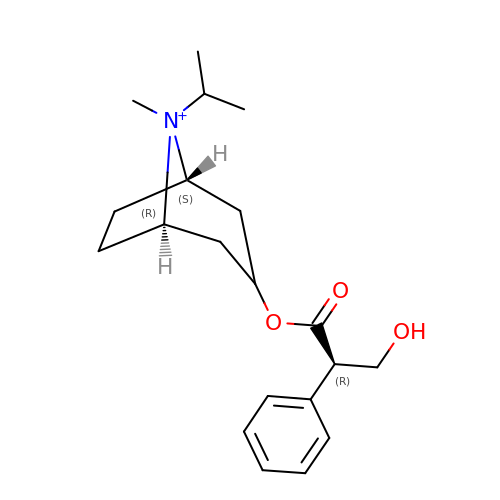IPRATROPIUM | C20 H30 N O3 | OEXHQOGQTVQTAT-KKKDIUQISA-N>MASDGVVVEIGKVTGSVGTTVEIPVYFRGVPSKGIANCDFVFRYDPNVLEIIGIDPGDIIVDPNPTKSFDTAIYPDRKIIVFLFAEDSGTGAYAITKDGVFAKIRATVKSSAPGYITFDEVGGFADNDLVEQKVSFIDG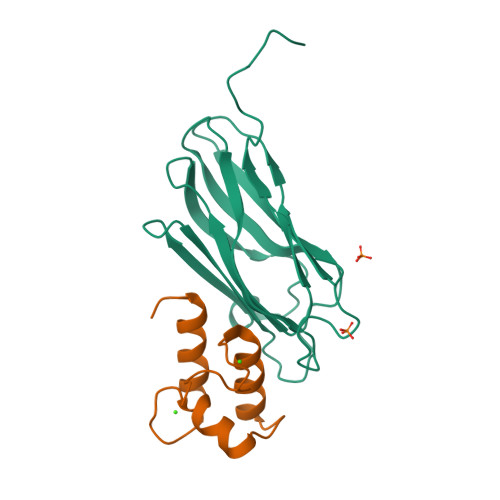GVNVGNATPTKLEHHHHHH[2x];>[2x]MVLLGDVNGDGTINSTDLTMLKRSVLRAITLTDDAKARADVDKNGSINAADVLLLSRYLLRVI3-azanyl-4-(7-fluoranyl-2H-indazol-4-yl)-8-methoxy-1H-1,5-naphthyridin-2-one | C16 H12 F N5 O2 | 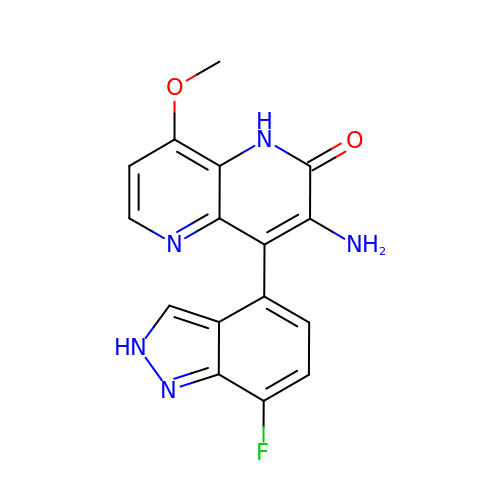CMDVDQKZWRQICJ-UHFFFAOYSA-N> GLPVLNTPGSNQYLTADNYQSPCAIPEFDVTPPIDIPGEVRNMMELAEIDTMIPLNLTNQRKNTMDMYRVELNDAAHSDTPILCLSLSPASDPRLAHTMLGEILNYYTHWAGSLKFTFLFCGSMMATGKLLVSYAPPG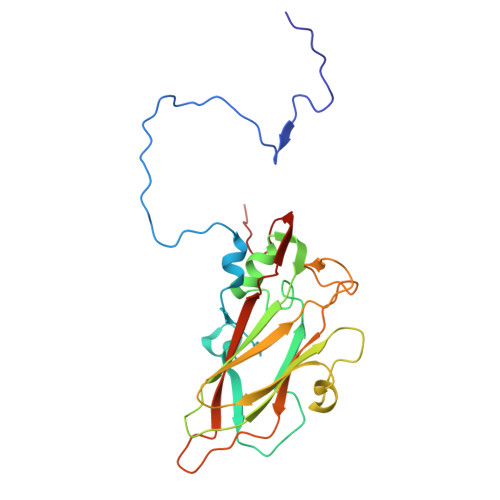AEAPKSRKEAMLGTHVIWDIGLQSSCTMVVPWISNTTYRQTINDSFTEGGYISMFYQTRVVVPLSTPRKMDILGFVSACNDFSVRLLRDTTHISQEA(1~{S},6~{R})-6-[(1-methoxycarbonyl-3,4-dihydro-2~{H}-quinolin-6-yl)carbamoyl]cyclohex-3-ene-1-carboxylic acid | C19 H22 N2 O5 | 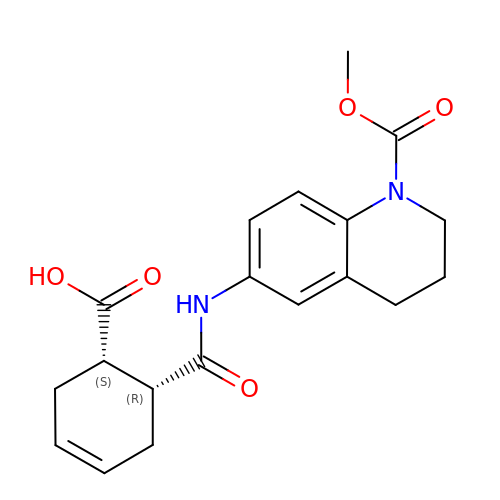KPFUFQIEFZZIBO-CABCVRRESA-N>MIDRRFGVAAAALALLAACSSPPSARSAPTQLPTAAPGTASASTPHALLLISIDGLRADMLDRGITPNLSHLAREGVRARWMAPSYPSLAFPNHYTLVTGLRPDHHGIVHNSMRDPTLGGFWLSKSEAVGDARWWGGEPVWVGVENTGQHAATWSWPGSEAAIKGVRPSQWRHYQKGVRLDTRVDAVRGWLATDGAQRNRLVTLYFEHVDEAGHDHGPESRQYADAVRAVDAAIGRLLAGMQRDGTRARTNIIVVSDHGMAEVAPGHAISVEDIAPPQIAT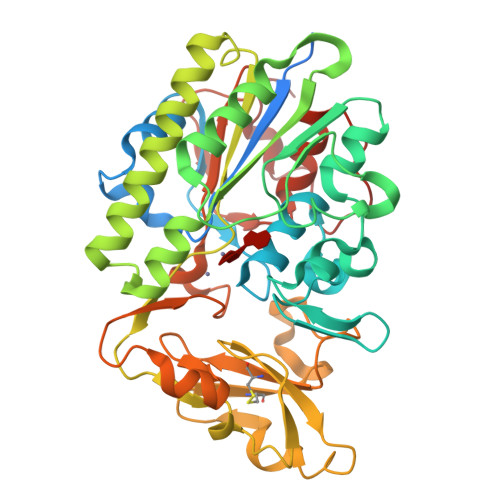AITDGQVIGFEPLPGQQAAAEASVLGAHDHYDCWRKAELPARWQYGSHPRIPSLVCQMHEGWDALFPDKLAKRAQRGTRGSHGYDPALPSMRAVFLAQGPDLAQGKTLPGFDNVDVYALMSRLLGIPAAPNDGNPATLLPALRMPP[6x]>MAKDKEFQVLFVLTILTLISGTIFYSTVEGLRPIDALWFSVVTLTTVGYGDFSPQTDFGKIFTILYIFIGIGLVFGFIHKLAVNVQLPSILSNL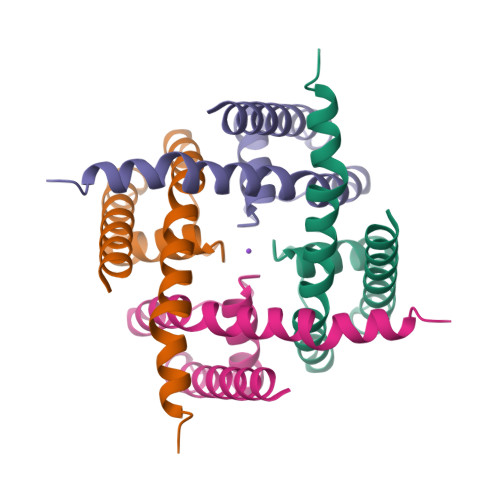VPR[2x]> AVTGTTKANIKLFSFTEVNDTNPLNNLNFTLKNSGKPLVDMVVLFSANINYDAANDKVFVSNNPNVQHLLTNRAKYLKPLQDKGIKVILSILGNHDRSGIANLSTARAKAFAQELKNTCDLYNLDGVFFDDEYSAYQTPPPSGFVTPSNNAAARLAYETKQAMPNKLVTVYVYSRTSSFPTAVDGVNAGSY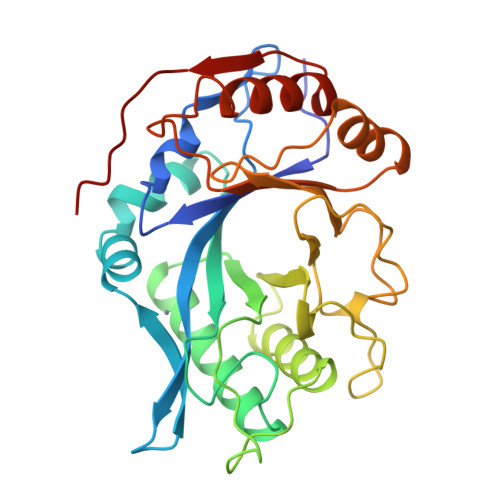VDYAIHDYGGSYDLATNYPGLAKSGMVMSSQEFNQGRYATAQALRNIVTKGYGGHMIFAMDPNRSNFTSGQLPALKLIAKELYGDELVYSNTPYSKDW> EPVQFKDCGSVDGVIKEVNVSPCPTQPCQLSKGQSYSVNVTFTSNIQSKSS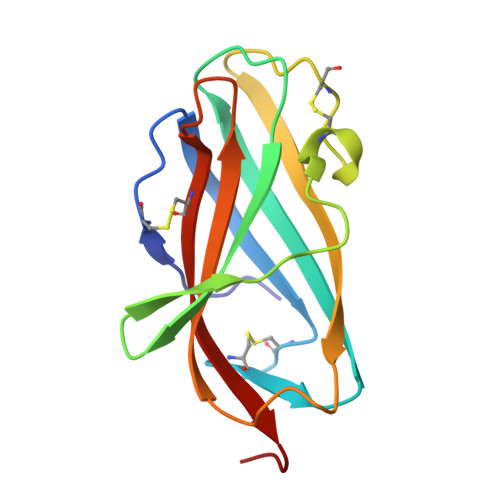KAVVHGILMGVPVPFPIPEPDGCKSGINCPIQKDKTYSYLNKLPVKSEYPSIKLVVEWQLQDDKNQSLFCWEIPVQIVSHLA> PVTLEPMPPGEGAQEGEPPTVEARYKSFSIKMLKDMKEGVKQYGPNSPYMRTLLDSIAHGHRLIPYDWEILAKSSLSPSQFLQFKTWWIDGVQEQVRRNRAANPPVNI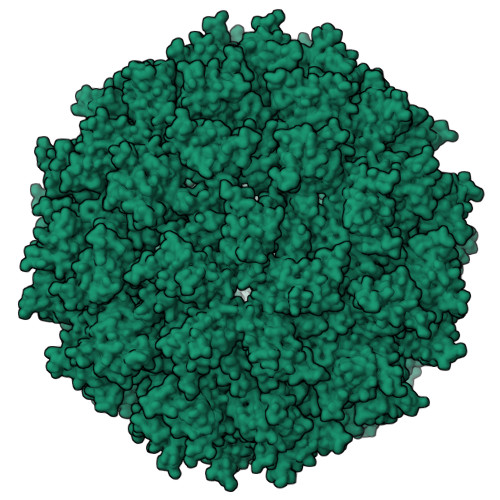DADQLLGIGQNWSTISQQALMQNEAIEQVRAICLRAWEKIQDPGSACPSFNTVRQGSKEPYPDFVARLQDVAQKSIADEKARKVIVELMAYENANPECQSAIKPLKGKVPAGSDVISEYVKACDGIGGAMHKAMLMAQLE>MEAVPRMPMIWLDLKEAGDFHFQPAVKKFVLKNYGENPEAYNEELKKLELLRQNAVRVPRDFEGCSVLRKYLGQLHYLQSRVPMGSGQEAAVPVTWTEIFSGKSVAHEDIKYEQACILYNLGALHSMLGAMDKRVSEEGMKVSCTHFQCAAGAFAYLREHFPQAYSVDMSRQILTLNVNLMLGQAQECLLEKSMLDNRKSFLVARISAQVVDYYKEACRALENPDTASLLGRIQKDWKKLVQMKIYYFAAVAHLHMGKQAEEQQKFGERVAYFQSALDKLNEAIKLAKGQPDTVQDALRFTMDVIGGKYNSAKKDNDFIYHE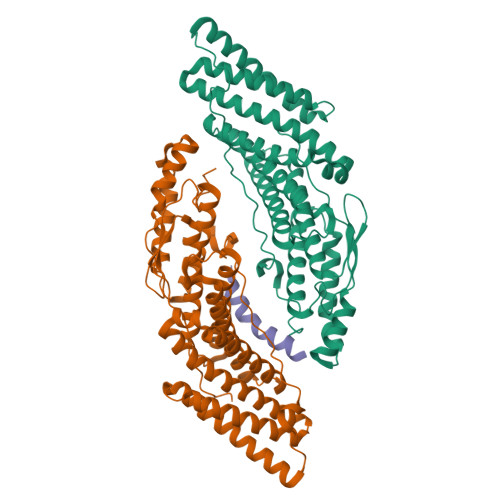AVPALDTLQPVKGAPLVKPLPVNPTDPAVTGPDIFAKLV[4x];>[2x]MENYFQAEAYNLDKVLDEFEQN>[2x]ARKDNLAKTIAETAKIREVLI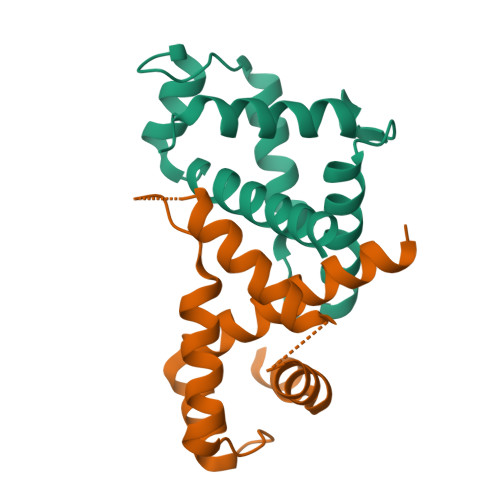IQNVLNCFNDDQVRSDFLNGENGAKKLENTELELLEKFFIETQTRRPETADDVSFIATAQKSAELFYSTINARPKSFGEVSFEKLRSLFQQIQDSGYLDKYYL> MRYKKKWAATEPKFPAVRLALQNFDMTYSVQFGDLWPSIRVSLLSEQKYGALVNNFAAWDHVSAKLEQLSAKDFVNEAISHWELQSEGGQSAAPSPASWACSPNLRCFTFDRGDISRFPPARPGSLGVMEYYLMDAASLLPVLALGLQPGDIVLDLCAAPGGKTLALLQTGCCRNLAANDLSPSRIARLQKILHSYVPEEIRDGNQVRVTSWDGRKWGELEGDTYDRVLVDVPCTTDRHSLHEEENNIFKRSRKKERQILPVLQVQLLAAGLLATKPGGHVVYSTCSLSHLQNEYVVQGAIELLANQYSIQVQVEDLTHFRRVF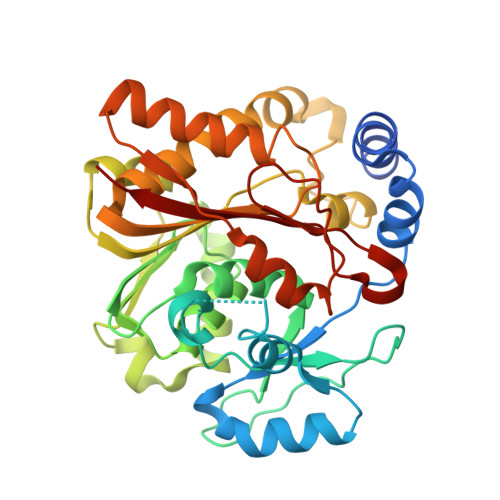MDTFCFFSSCQVGELVIPNLMANFGPMYFCKMRRLT>GSMAQILPIRFQEHLQLQNLGINPANIGFSTLTMESDKFICIREKVGEQAQVVIIDMNDPSNPIRRPISADSAIMNPASKVIALKAGKTLQIFNIEMKSKMKAHTMTDDVTFWKWISLNTVALVTDNAVYHWSMEGESQPVKMFDRHSSLAGCQIINYRTDAKQKWLLLTGISAQQNRVVGAMQLYSVDRKVSQPIEGHAASFAQFKMEGNAEESTLFCFAVRGQAGGKLHIIEVGTPPTGNQPFPKKAVDVFFPPEAQNDFPVAMQISEKHDVVFLITKYGYIHLYDLETGTCIYMNRISGETIFVTAPHEATAGIIGVNRKGQVLSVCVEEENIIPYITNVLQNPDLALRMAVRNNLAG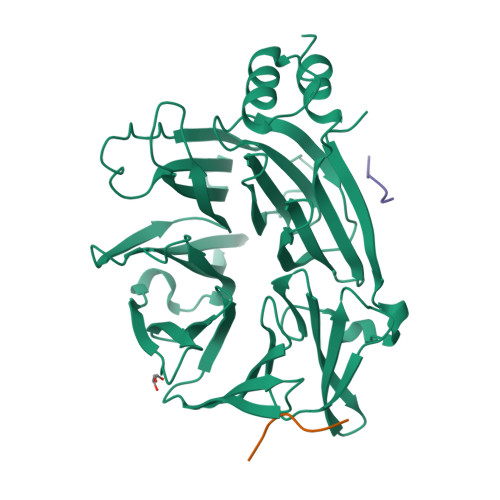AEEL[2x];>SDILFPADS[4x]> MTMAANTDRAVLQAALPPLSGSLPIPGLSASVRVRRDAWGIPHIKASGEADAYRALGFVHSQDRLFQMELTRRKALGRAAEWLGAEAAEADILVRRLGMEKVCRRDFEALGVEAKDMLRAYVAGVNAFLASGAPLPVEYGLLGAEPEPWEPWHSIAVMRRLGLLMGSVWFKLWRMLALPVVGAANALKLRYDDGG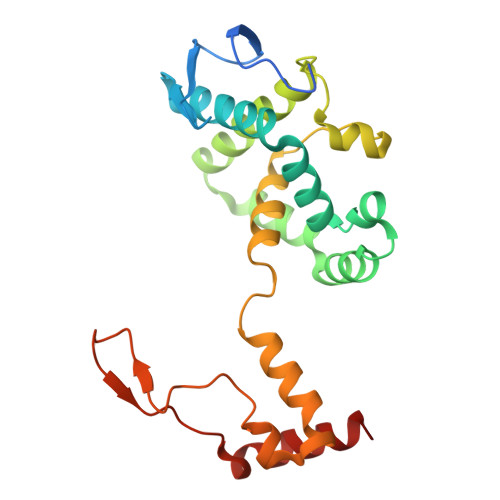RDLLCIPPGAEADRLEADLATLRPAVDALLKAMG>MVTLHLAHLTLTHAQPSYAALECIPAMQRRRLSPLAKLALNTAISSLDGRSADYIVWVSKYGDEAKTLNILQDVLNDQTPSPTQFSTSVHNAISGLYSILCQDDTPSTSLSCSWTEGLIEAYALLKSMPEIKRVLVVAYDEPLPNIYAEAINFPAYAMAAVVTLEQPNLQITAWTHTDEAEAPAFAHFWQDADQLTSAFGWNKC[2x];>[2x]MKHLPSENAAPMAVGIQFSVGLSALGCELNQIKQALQQPQQTLSLRDDLIADRDVWVGQYTHPLCSSVPDAMRSVDSRNLRFALTALSKIETELKAYTASFENKRLAIVVGTSTSGIADNELLLKQYFQGQTDLSISHYPQEMSCLAKALQQYLGWEGPAYTISTACSSSAKALAAGQRLLHADLADV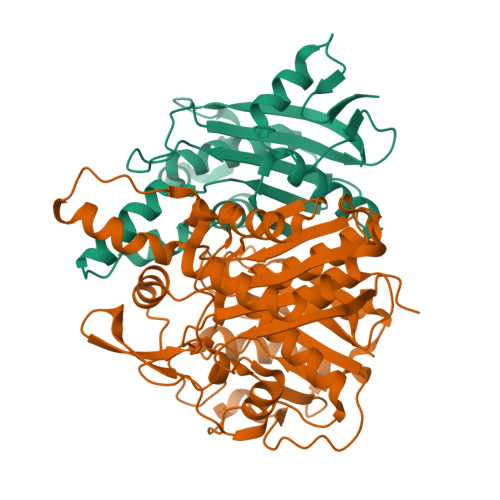VLVGGVDTLCKLTLNGFNSLESLSAHICQPCGISRDGINIGEAAAFFVLSKEQAPVMLMGAGETMDAWHISAPHPEGKGAALAMQRALDMAHISAQEVGYINLHGTATPQNDAMEIKAVRQVFGVYQVALSSTKHKTGHCLGAAGAIEAFICEQVLKDQSWLPLHQNVEIDPDLVDQNYVQEAELTQPIRYVMSNSFAFGGSNISLVFGVKP> HHHHHHHFELCDAVSGEKIPAATQNTNTNSNRYEGKVIDSAPLLPKMDFKSSPFRMYKVGTEFLVYDH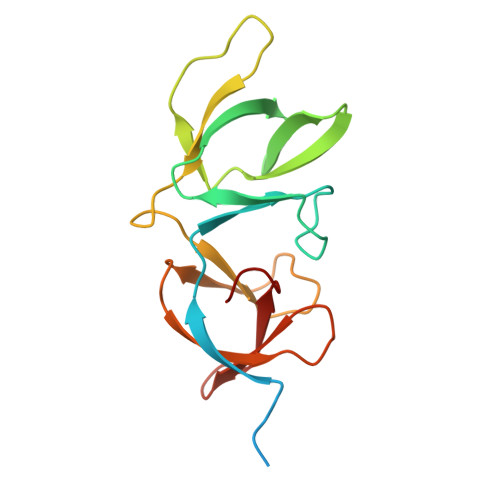NQYWYKTYIDDKLYYMYKSFCDVVAKKDAKGRIKVRIKSAKDLRIPVWNNIKLNSGKIKWYAPNVKLAWYNYRRGYLELWYPNDGWYYTAEYFLK> QLYEN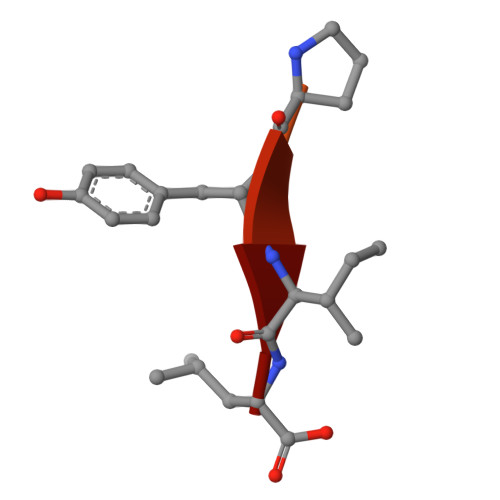KPRRPYIL> SMHLICQSGDVLSARYEIVDTLGEGAFGKVVECIDHKAGGRHVAVKIVKNVDRYCEAARSEIQVLEHLNTTDPNSTFRCVQMLEWFEHHGHICIVFELLGLSTYDFIKENGFLPFRLDHIRKMAYQICKSVN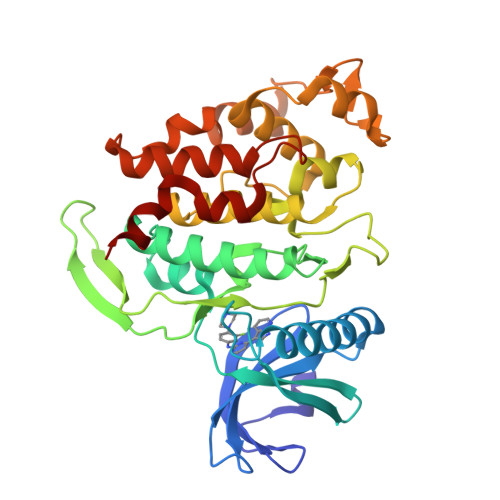FLHSNKLTHTDLKPENILFVQSDYTEAYNPKIKRDERTLINPDIKVVDFGSATYDDEHHSTLVSTRHYRAPEVILALGWSQPCDVWSIGCILIEYYLGFTVFPTHDSKEHLAMMERILGPLPKHMIQKTRKRKYFHHDRLDWDEHSSAGRYVSRACKPLKEFMLSQDVEHERLFDLIQKMLEYDPAKRITLREALKHPFFDLLKKSI> SAPSPQSPETPAPQNQTSRVVQAPKEEEEDEQEASEEKASEEEKAWLMASRQQLAKETSNFGFSLLRKISMRHDGNMVFSPFGMSLAMTGLMLGATGPTETQIKRGLHLQALKPTKPGLLPSLFKGLRETLSRNLELGLTQGSFAFIHKDFDVKETFFNLSKRYFDTECVPMNFRNASQAKRLMNHYINKETRGK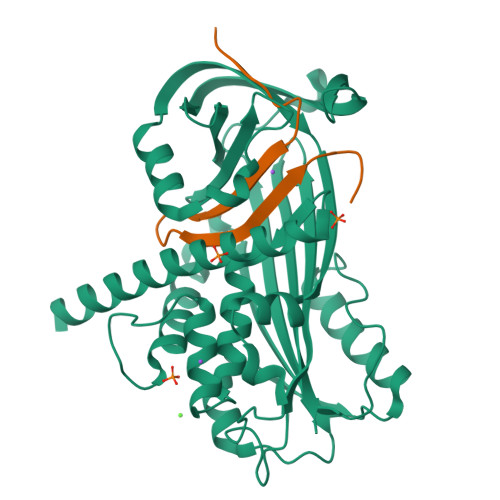IPKLFDEINPETKLILVDYILFKGKWLTPFDPVFTEVDTFHLDKYKTIKVPMMYGAGKFASTFDKNFRCHVLKLPYQGNATMLVVLMEKMGDHLALEDYLTTDLVETWLRNMKTRNMEVFFPKFKLDQKYEMHELLRQMGIRRIFSPFADLSELSATGRNLQVSRVLQRTVIEVDERGTEAVAGILSEITAR;> SMPPVIKIDRPFHFMIYEETSGMLLFLGRVVNPTLL>MAQFPNTPSFTGFNTPSRIEADIADLAHEGTIPQGLNGAFYRVQPDPQFPPRLDDDIAFNGDGMITRFHIHDGQVDFRQRWAKTDKWKLENAAGKALFGAYRNPLTDDEAVKGEIRSTANTNAFVFGGKLWAMKEDSPALVMDPATMETFGFEKFGGKMTGQTFTAHPKVDPKTGNMVAIGYAASGLCTDDVTYMEVSPEGELVREVWFKVPYYCMMHDFGITEDYLVLHIVPSIGSWERLEQGKPHFGFDTTMPVHLGIIPRRDGVRQEDIRWFTRDNCFAFHVLNAW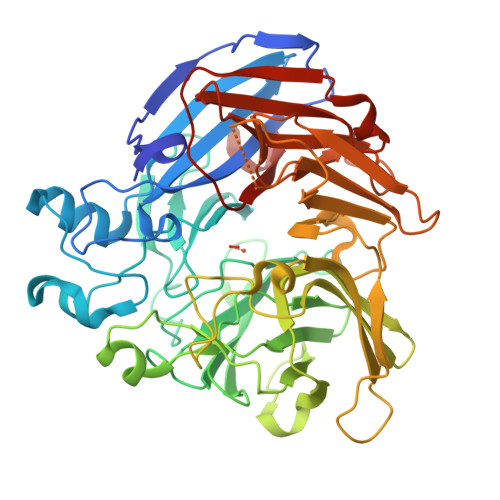QEGTKIHFVTCEAKNNMFPFFPDVHGAPFNGMEAMSHPTDWVVDMASNGEDFAGIVKLSDTAAEFPRIDDRFTGQKTRHGWFLEMDMKRPVELRGGSAGGLLMNCLFHKDFETGREQHWWCGPVSSLQEPCFVPRAKDAPEGDGWIVQVCNRLEEQRSDLLIFDALDIEKGPVATVNIPIRLRFGLHGNWANADEIGLAEKVLAA[3x]> MTQVASPVVQARYSPVELSAALGLFPPTDEQAAVIAAPPGPLVVIAGAGAGKTETMAARVVWLVANGFATPSQVLGLTFTRKAAGQLLRRVRTRLARLAGAGLAPGSGASDESATVSTYHAFAGTLLREHGLLLPVEPDTRLLSETELWQLAYDVVCAHPGHLDTEKTPAAVTAMVLRLSGALAEHLVDTDQLRDTHVELERLVHTLPAGPYQRDRGPSQWLLRMLATQTERTELVPLIDALHQRMRAEKVMDFGMQMAAAARLAARFPQVGEQLRQRFRVVLLDEYQDTGHAQRIALSSLFGGGADDGLALTAVGDPIQSIYGARGASATNLPRFTTDFPYSDGTPAPTLELRTSWRNPPSTLHVANAVSEEARRRSVAVRALRPRPDAEPGTIRCALLNNVAAERDWVADHLARAYHGAIGRGEAAPTAAVLVRRNADAAPMAEALTARGVPVEVVGVAGLLAVPEVADLVAMLRLIADPTAGSAVMRILTGPRWRFGARDIAALWRRAVELDDRPKGELGTADIVAQAAPDADTACVADAICDPGDAERYSPAGYERIVALGRELTMLRAHLGHPLPELVAEVRRVLGLDAEARAARPVAAGWAGTENLDRFSDLVSDFAGHAGASVSALLAYLDAAVEVENGLAPAELTVSHDRVQILTVHAAKGLEWQVVAVPHLSARVFPSTTQARTWLTDASDLPP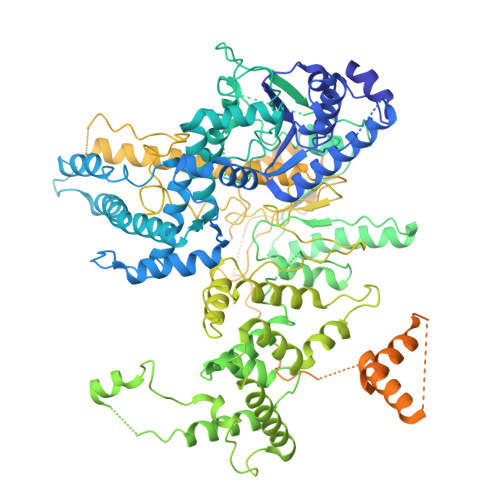LLRGDRATESEIGVPVLDTSDIYDRKILSDKISDHKKSLDQRRVDEERRLLYVAITRAEDTLLLSGHHWGATESKPRGPSEFLCELKTILEEATAAGTPCGEIEHWAPDPAPGETNPLRDQVVEALWPPVASADDHVHRGAQLVAAAMAGEVSAEADQEGWAADVDALLAERERPPQQEDTELPGQLSVSTLVELSRDPKAALTRLRRRLPQRPDPHALLGTTFHEWVQRYFHAERLFDLDDLPGAVDSDSGRAVEESLAELQDAFVKSPWAARTPVEVEVPFDMVLGETVVRGRIDAVFAEPDGTTMVLDWKTGDPPETPEAKEHAAVQLAVYRLAWAAMRGCPPESVRAAFHYVRSGQTVIPETLPGAEELVKLLAAAPTETAEEADRIT>MATKGTKRSYEQMETDGERQNATEIRASVGKMIDGIGRFYIQMCTELKLSDYEGRLIQNSLTIERMVLSAFDERRNKYLEEHPSAGKDPKKTGGPIYRRVDGKWRRELILYDKEEIRRIWRQANNGDDATAGLTHMMIWHSNLNDATYQRTRALVRTGMDPRMCSLMQGSTLPRRSGAAGAAVKGVGTMVMELIRMIKRGINDRNFWRGENGRRTRIAYERMCNILKGKFQTAAQRTMVDQVRESRNPGNAEFEDLIFLARSALILRGSVAHKSCLPACVYGSAVASGYDFEREGYSLVGIDPFRLLQNSQVYSLIRPNENPAHKSQL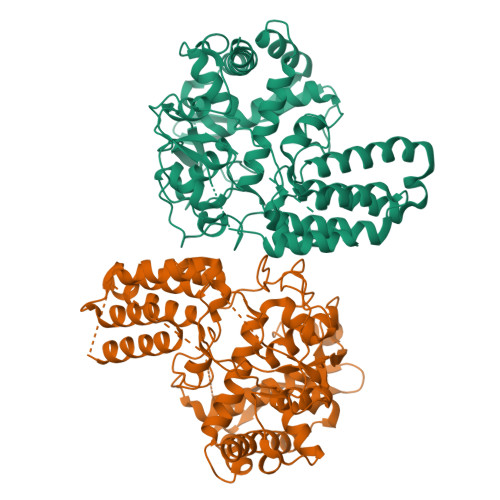VWMACHSAAFEDLRVSSFIRGTKVVPRGKLSTRGVQIASNENMETMESSTLELRSRYWAIRTRSGGNTNQQRAGGGGSTGNTEGRTSDMRTEIIRLMESARPEDVSFQGRGVFELSDEKATSPIVPSFDMSNEGSYFFGDNAEEYDNLEHHHHHH[2x]>[3x]MKGDAKVIEFLNAALRSELTAISQYWVHFRLQEDWGLAKMAKKSREESIEEMGHADKIIARILFLEGHPNLQKLDPLRIGEGPRETLECDLAGEHDALKLYREARDYCAEVGDIVSKNI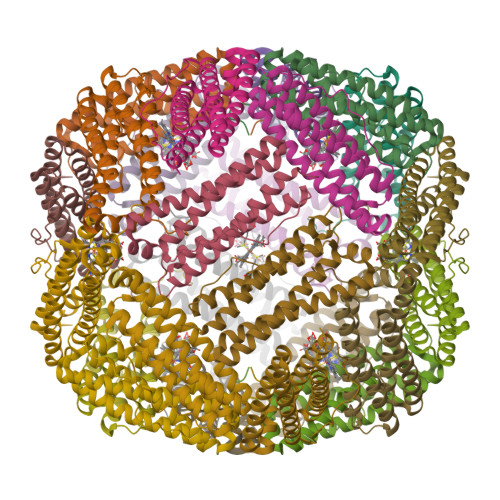FESLITDEEGHVDFLETQISLYDRLGPQGFALLNAAPMDAAE> DADKIEDEVTRQVAQCKCAKRFQVEQIGENKYRFGDSQQLRLVRILRSTVMVRVGG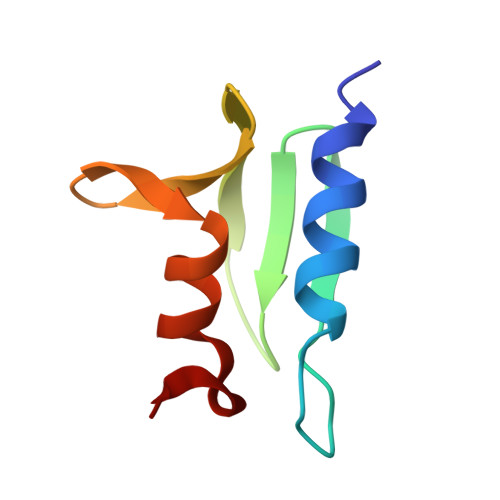GWMALDEFLVKNDPCRAR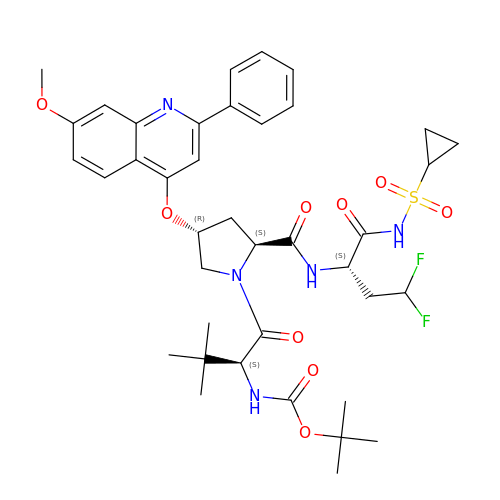N-(tert-butoxycarbonyl)-3-methyl-L-valyl-(4R)-N-{(2S)-1-[(cyclopropylsulfonyl)amino]-4,4-difluoro-1-oxobutan-2-yl}-4-[(7-methoxy-2-phenylquinolin-4-yl)oxy]-L-prolinamide | C39 H49 F2 N5 O9 S | LGOOHMFDMLUYDW-RXAGJDKHSA-N>MSKKILQLTDDSFELNVISASGVVLVDFWAEWCSPCKSISPIIDEISIEYADKLTVGKLNIDQNPVVPTKYGIRSIPTLLLFKSGEVIATKVGALSKAQLREFLDAYL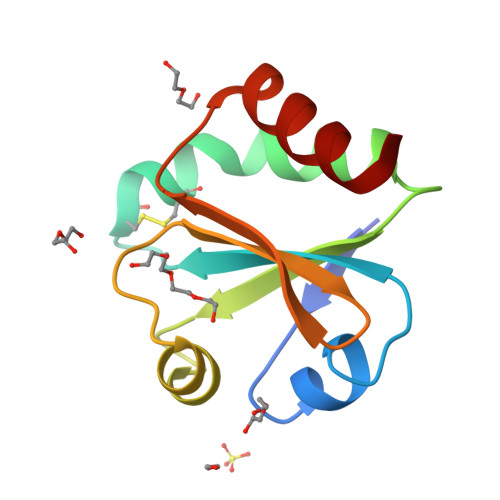K[2x]Computational design of KE07 involved construction of a theozyme to catalyze the chemical reaction, which was then grafted into the scaffold of imidazole glycerol phosphate synthase (HisF) from Thermotoga maritima. Catalytically essential residues from the initial design include a base (Glu101) that facilitates C−H bond cleavage, an H-bond donor (Lys222) to stabilize the phenoxide intermediate, and a π-stacking residue (Trp50), which was designed to stabilize the transition state and favor substrate binding through interactions with the aromatic ring of the substrate. This initial KE07 design (Round 1; R1) catalyzes the cleavage of 5-nitrobenzisoxazole, with 103-fold rate acceleration over the noncatalyzed reaction and a turnover rate (kcat) of 0.018 s−1.

The mutations in R7 and R7-2 (Phe77Ile, Phe229Ser, Ile102Phe) result in further optimization of activation energy. Finally, crystals of R7-2 with the hexahistidine tag crystallized in configuration B with the hexahistidine tag in the active site (even when soaked with substrate). However, when we removed the hexahistidine tag, we captured a high-resolution structure in configuration C with product bound (configuration A was present in low occupancy). However, in later generations (R7 and R7-2) evidence for turnover was only observed with configuration C. By R7 and R7-2, configuration C (which was the only state we saw associated with product in the crystal structures) becomes the dominant substate sampled, with configurations A and B sampled only rarely. In the most evolved versions of the three configurations we obtained from our structural studies (R7, A; R7-2, B; R7-2, C), configurations B and C displayed lower energy barriers than A (16.8 and 16.4 vs. 19.0 kcal mol−1, respectively), which is consistent with the gradual conformational selection of state C along the trajectory.

> MALAKRIDAALIMKDGRVVKGSNFENLRDSGDPVELGKFYSEIGIDELSFWDITASVEKRKTMLELVEKVAEQIDIPITVGGGIHDFETASELILRGADKVEFNTAAVENPSLITQIAQTFGSQAVVVYIAAKRVDGEFMVFTYSGTKNTGILLRDWVVEVEKRGAGEIVLGSIDRLGTKSGYDTEMIRFVRPLTTLPIIAHRGAGKMEHFLEAFLAGADAAKADSVFHSREIDVRELKEYLKKHGVNVRLEGLGSLEHHHHHH>XPPGPPGPPGPPGPPGPRGPPGXGPPGPPGPP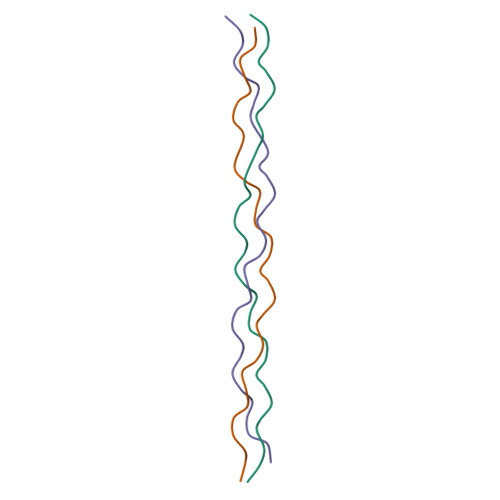G[3x]8-(4-azanylbutyl)-6-[2-chloranyl-5-(trifluoromethyl)phenyl]-2-(methylamino)pyrido[2,3-d]pyrimidin-7-one 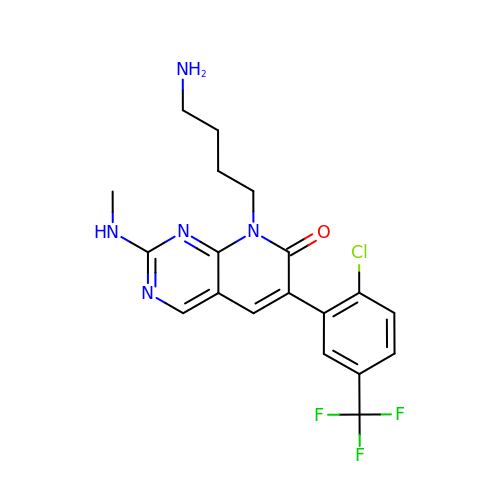| C19 H19 Cl F3 N5 O | HWGFCLUXIWWFKE-UHFFFAOYSA-N>STGDVTLTKTDATTKAALAGAVYELQDATGKVLKMGLTTDTTGQLTVSGLTAGNYQFVETKAPSGYQLNAA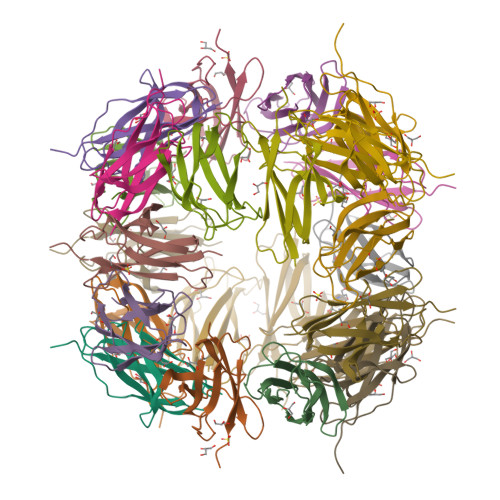PLSFTIKPNQTAVVTVAATDEPVTEPG[12x]N'-(6-aminopyridin-3-yl)-N-(2-cyclopentylethyl)-4-methyl-benzene-1,3-dicarboxamide | C21 H26 N4 O2 | 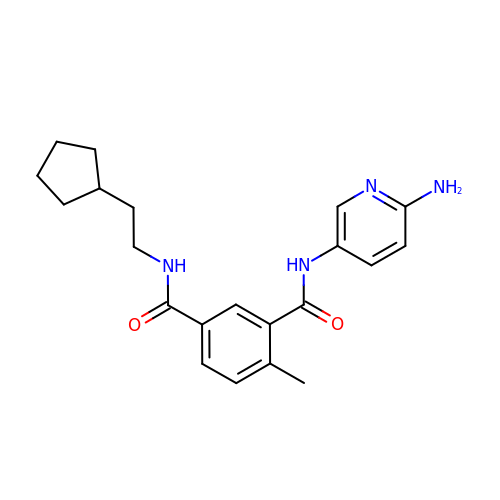CLEGTVIMOPPIBR-UHFFFAOYSA-N> DRVYIHPFHLLYYSKSTCAQLENPSVETLPEPTFEPVPIQAKTSPVDEKTLRDKLVLATEKLEAEDRQRAAQVAMIANFVGFRMYKMLSEARGVASGAVLSPPALFGTLVSFYLGSLDPTASQLQVLLGVPVKEGDCTSRLDGHKVL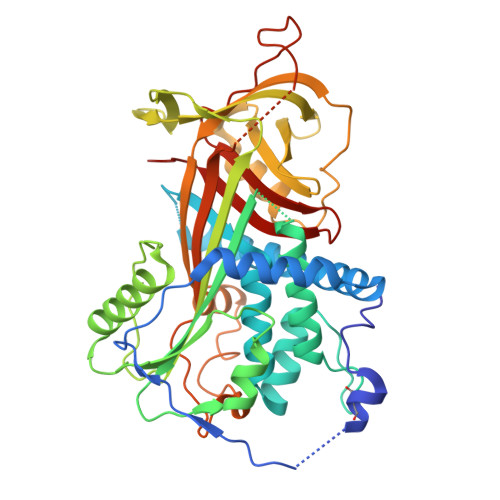TALQAVQGLLVTQGGSSSQTPLLQSTVVGLFTAPGLRLKQPFVESLGPFTPAIFPRSLDLSTDPVLAAQKINRFVQAVTGWKMNLPLEGVSTDSTLFFNTYVHFQGKMRGFSQLTGLHEFWVDNSTSVSVPMLSGTGNFQHWSDAQNNFSVTRVPLGESVTLLLIQPQCASDLDRVEVLVFQHDFLTWIKNPPPRAIRLTLPQLEIRGSYNLQDLLAQAKLSTLLGAEANLGKMGDTNPRVGEVLNSILLELQAGEEEQPTESAQQPGSPEVLDVTLSSPFLFAIYERDSGALHFLGRVDNPQNVV;> DRVYIHPFHLLYYSKSTCAQLENPSVETLPEPTFEPVPIQAKTSPVDEKTLRDKLVLATEKLEAEDRQRAAQVAMIANFMGFRMYKMLSEARGVASGAVLSPPALFGTLVSFYLGSLDPTASQLQVLLGVPVKEGDCTSRLDGHKVLTALQAVQGLLVTQGGSSSQTPLLQSTVVGLFTAPGLRLKQPFVESLGPFTPAIFPRSLDLSTDPVLAAQKINRFVQAVTGWKMNLPLEGVSTDSTLFFNTYVHFQGKMRGFSQLTGLHEFWVDNSTSVSVPMLSGTGNFQHWSDAQNNFSVTRVPLGESVTLLLIQPQCASDLDRVEVLVFQHDFLTWIKNPPPRAIRLTLPQLEIRGSYNLQDLLAQAKLSTLLGAEANLGKMGDTNPRVGEVLNSILLELQAGEEEQPTESAQQPGSPEVLDVTLSSPFLFAIYERDSGALHFLGRVDNPQNVV>[2x]GHMRKLKIGITCYPSVGGSGIIATELGKQLAEKGHEIHFITSSIPFRLNTYHPNIHFHEVEVNQYAVFKYPPYDLTLASKIAEVAERENLDIIHAHYALPHAVCAYLAKQMLKRNIGIVTTLHGTDITVLGYDPSLKDLIRFAIESSDRVTAVSSALAAETYDLIKPEKKIETIYNFIDERVYLKKNTAAIKEKHGILPDEKVVIHVSNFRKVKRVQDVIRVFRNIAGKTKAKLLLVGDGPEKSTA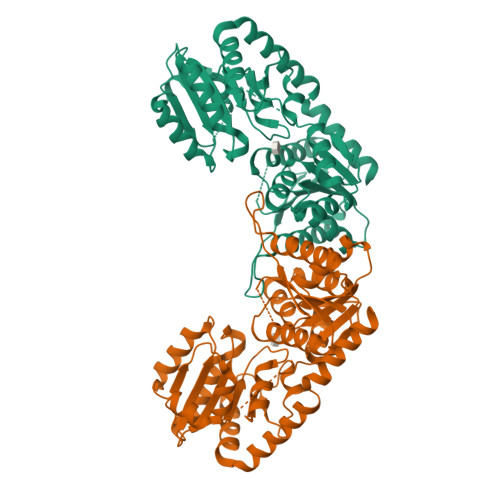CELIRKYGLEDQVLMLGNQDRVEDLYSISDLKLLLSEKESFGLVLLEAMACGVPCIGTNIGGIPEVIKNNVSGFLVDVGDVTAATARAMSILEDEQLSNRFTKAAIEMLENEFSSKKIVSQYEQIYADLAEPE> DDHSELLVNTKSGKVMGTRVPVLSSHISAFLGIPFAEPPVGNMRFRRPEPKKPWSGVWNASTYPNNCQQYVDEQFPGFSGSEMWNPNREMSEDCLYLNIWVPSPRPKSTTVMVWIYGGGFYSGSSTLDVYNGKYLAYTEEVVLVSLSYRVGAFGFLALHGSQEAPGNVGLLDQRMALQWVHDNIQFFGGDPKTVTIFGESAGGASVGMHILSPGSRDLFRRAILQSGSPNCPWASVSVAEGRRRAVELGRNLNCNLNSDEELIHCLREKKPQELIDVEWNVLPFDSIFRFSFVPVIDGEFFPTSLESMLNSGNFKKTQILLGVNKDEGSFFLLYGAPGFSKDSESKISREDFMSGVKLSVPHANDLGLDAVTLQYTDWMDDNNGIKNRDGLDDIVGDHNVICPLMHFVNKYTKFGNGTYLYFFNHRASNLVWPEWMGVIHGYEIEFVFGLPLVKELNYTAEEEALSRRIMHYWATFAKTGNPNEPHS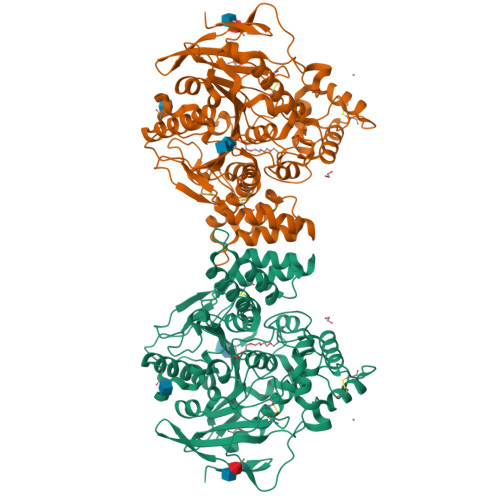QESKWPLFTTKEQKFIDLNTEPMKVHQRLRVQMCVFWNQFLPKLLNATAC> LAAKEAKLRDLEDSLARERDTSWRLLAEKE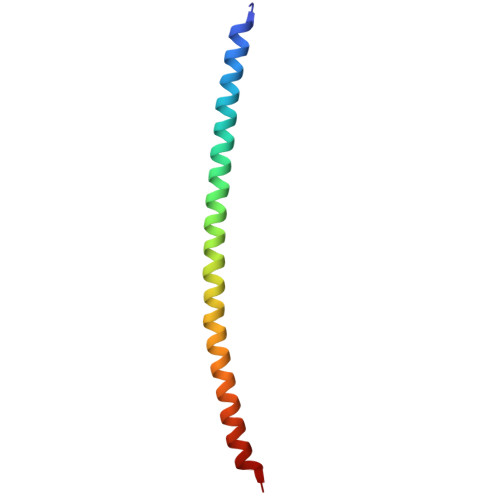REMAEMRARMQQQLDEYQELLDIKLALDMEIHAYRKLLEGEEER> SMSLNIITVTLNMEKYNFLGISIVGQSNERGDGGIYIGSIMKGGAVAADGRIEPGDMLLQVNDMNFENMSNDDAVRVLRDIVHKPGPIVLTVAKC

The central event in Wnt-PCP pathway is the activation of Weak-similarity guanine nucleotide exchange factor (WGEF) by the adapter protein Dishevelled (Dvl). The PDZ domain of Dishevelled2 (Dvl2PDZ) binds and activates WGEF by releasing it from its autoinhibitory state. Dvl2PDZ binds to both C-terminal as well as the non-canonical internal peptides. Using biochemical and molecular dynamics studies, we show that a unique “internal-PDZ binding motif” (IPM) of WGEF mediates the WGEF-Dvl2PDZ interaction to activate the GEF.

Additionally, the apo structure of human Dvl2PDZ shows conformational dynamics different from its IPM peptide bound state, suggesting an induced fit mechanism for the Dvl2PDZ-peptide interaction. A comparison of available Dvl2PDZ structures shows deviations with RMSD values in the range of 1.7–2 Å. Importantly, significant conformational variations are observed in the α2 helix and β2–β3 loop, which are part of the peptide binding pocket. This conformational variation is more prominent in the structures of human Dvl2PDZ, bound with different peptides. Interestingly, Sector 1 of apo Dvl2PDZ is composed of residues residing in β2 and α2 regions of the domain, whereas Sector 1 of Dvl2PDZ internal peptide (WGEFpep, WGEFpepQ8A and N3pep) complexes had residues from the β2 strand, β1–β2 and β2–β3 loops. Additionally, variations in Sector 1 composition highlight peptide-dependent conformational adaptation of Dvl2PDZ domain. In contrast to the earlier study by Munz et al., we observe that the α2 helix of the apo Dvl2PDZ structure has limited conformational flexibility rather than having the ability to explore all possible conformational space, specific to the ligand-bound forms. Thus, our structural and MD simulation studies suggest that Dvl2PDZ adopts peptide-dependent conformational change due to its intrinsic flexibility. In short, we can infer that Dvl2PDZ may not have a preformed binding pocket, rather it modulates the binding pocket based on the substrate available for binding.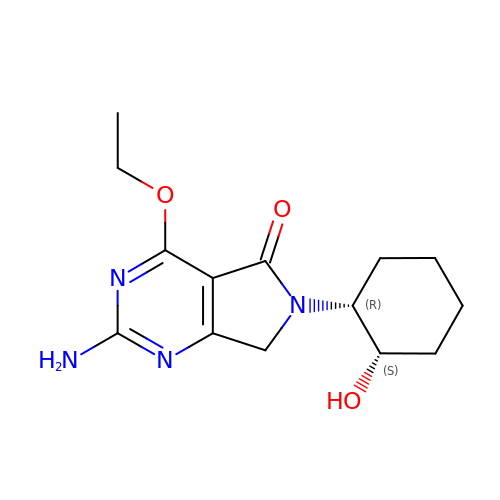2-azanyl-4-ethoxy-6-[(1~{R},2~{S})-2-oxidanylcyclohexyl]-7~{H}-pyrrolo[3,4-d]pyrimidin-5-one | C14 H20 N4 O3 | BIALHCSDJYVDGR-ZJUUUORDSA-N>GPAAPAQSPAAPDPEASPLAEPPQEQSLAPWSPQTPAPPCSRCFARAIESSRDLLHRIKDEVGAPGIVVGVSVDGKEVWSEGLGYADVENRVPCKPETVMRIASISKSLTMVALAKLWEAGKLDLDIPVQHYVPEFPEKEYEGEKVSVTTRLLISHLSGIRHYGELYLREKFENSIESLRLFKNDPLFFKPGSQFLYSTFGYTLLAAIVERASGCKYLDYMQKIFHDLDMLTTVQEENEPVIYNRARFYVYNKKKRLVNTPY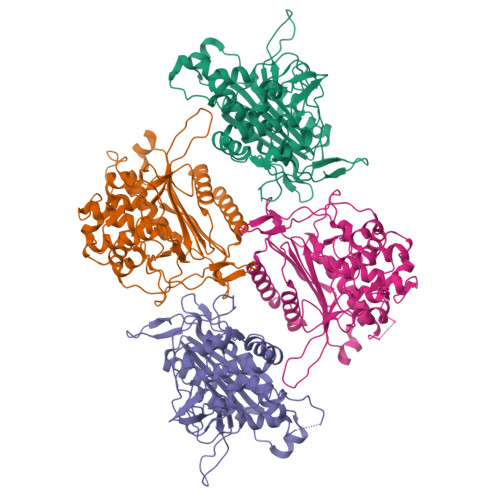VDNSYKWAGGGFLSTVGDLLKFGNAMLYGYQVGLFKNSNENLLPGYLKPETMVMMWTPVPNTEMSWDKEGKYAMAWGVVERKQTYGSCRKQRHYASHTGGAVGASSVLLVLPEELDTETINNKVPPRGIIVSIICNMQSVGLNSTALKIALEFDKDRSD[4x]> SLSCRPPMVKLVCPADNLRAEGLECTKTCQNYDLECMSMGCVSGCLCPPGMVRHENRCVALERCPCFHQGKEYAPGETVKIGCNTCVCQDRKWNCTDHVCDATCSTIGMAHYLTFDGLKYLFPGECQYVLVQDYCGSNPGTFRILVGNKGCSHPSVKCKKRVTILVEGGEIELFDGEVNVKRPMKDETHFEVVESGRYIILLLGKALSVVWDRHLSISVVLKQTYQEKVCGLCGNFDGIQNNDLTSSNLQVEEDPVDFGNSWKVSSQCADTRKVPLDSSPATCHNNIMKQTMVDSSCRILTSDVFQDCNKLVDPEPYLDVCIYDTCSCESIGDCACFCDTIAAYAHVCAQHGKVVTWRTATLCPQSCEERNLRENGYECEWRYNSCAPACQVTCQHPEPLACPVQCVEGCHAHCPPGKILDELLQTCVDPEDCPVCEVAGRRFASGKKVTLNPSDPEHCQICHCDVVNLTCEACQE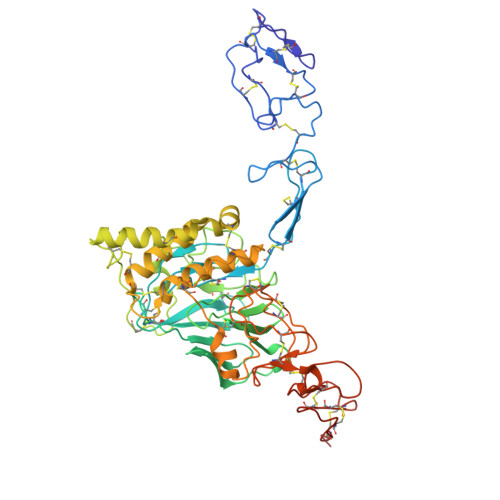PGGLVVPPHHHHHH> TQDRPLLAVQEALKKCFPVVEEQQGLWQSA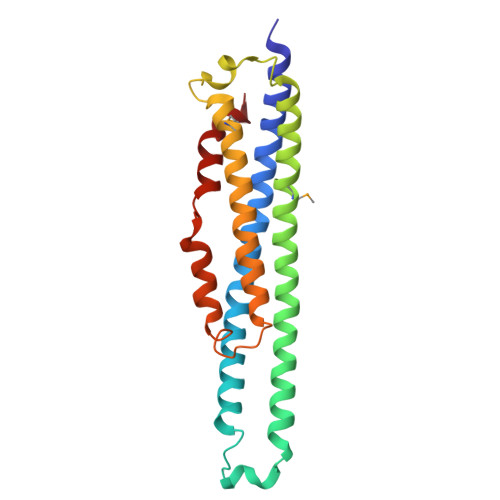LRDCQPLLSSLSNLAEQLQAAQNLRFEDVPALRAFPDLKERLRRKQLVAGDIVLDKLGERLAILLKVRDMVSSHVERVFQIYEQHADTVGIDAVLQPSAVSPSVADMLEWLQDIERHYRKSYLKRKYLLSSIQWGDLANIQALPKAWDRISKDEHQDLVQDILLNVSFFLEE> MKISQQQKLSLVNRTGKLEAKKESGQDGLCDVINFKTLKKGNWHSFKLQFDSKGATYGCLDQAGNVTLFYLDKNRYTNVDVQVDSSNLTFIEKPTGYLAVSNADCSISIYSILSGKLIQQLKWHTFKIKKLQVNHMSGYLLSVSSDNCTIWNINTYERRKSFFVKNTRYAQGCLTPAGEHLITLSQNGLVECHNTDTLKIEKKEEIGLKLKQAHLDISAEGVYIAICGDSNYCLIGRLDCQQGFDFELYELPNNIQSVKKIKFIRNSLLTLLGSDEKIYVLSAENNMEIVLCFELPSRKGIVDYDLNIDAKYLVVISTLGEKYVYDFHQLIANQKKHQQDVTMKKGSFSRQTLTRMDLDELKQTLFYQTKENQMKYANSKKQKHEGKINGETNMIMLDRVGGATPEVEIFVNGKRQDQYDIQNQKSSFLDREKLREFLSRFGYFPEKHRVVVWNYLLKLPSNYEAFDNLARKGLHPNYLNLKSTFPIQSDKLYYRTQRILSCLAHYCPVFAQLDYMPAFVFPFVKLLGTNEAFCFEVILSFLVQWGQFFFEFAPN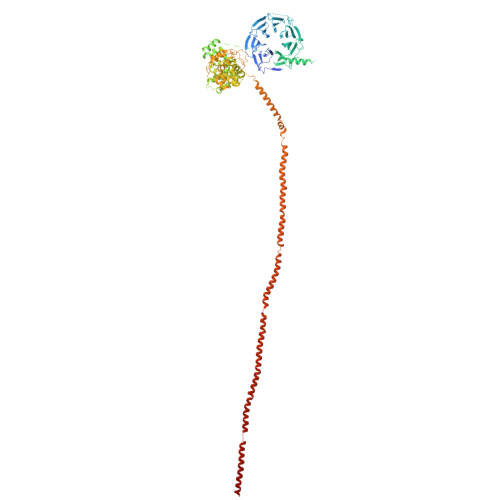PPVSYLKAFMELLEYHEPQLHAQLNQNIPHTQLFNTIWSSLQVVLTDVLKREDWLCFIDFLVAHSEKPDLLLHILVAYFTYFKRHIISFTTGSQLLRFFQQDHQIRIQNLLQDALEYRNRTPPRIPQAVVLQDNLPLTSEQYPIFNFYPKFSLDQHKEIREQIIQEELKATEKKRTLKELNTLQQQLNDLEKLYEEKQDALMRHERERREIITYEQEMRYSKLVDAERQVREERLQQMKKLEEESRKAIQIAENSRKADLDFIDQELQKKRANDNKFIASKMEEEAILNLELKTAGRINEVLNTKTKDQNIQSITLQAEIAQKRLDMKYKQMEQQIDQQIEEENIRQDHILQRKALQREIEDDVSKQREIKGQLLAEEFERE> GHMQETQAVEAGEKTVEQFVQALNKGDYNKAAEMTSKKAANKSALSEKEILDKYQNIYGAADVKGLQISNLKVDKKDDSTYSFSY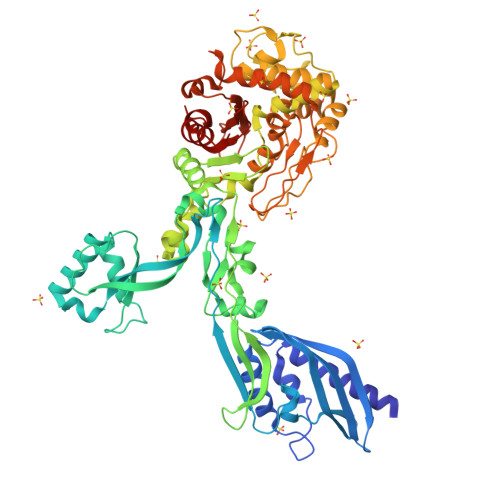KAKMNTSLGELKDLSYKGTLDRNDGQTTINWQPNLVFPEMEGNDKVSLTTQEAARGNIIDRNGEPLATTGKLKQLGVVPSKLGDGGEKTANIKAIASSFDLTEDAINQAISQSWVQPDYFVPLKIIDGATPELPAGATIQEVDGRYYPLGEAAAQLIGYVGDITAEDIDKNPELSSNGKIGRSGLEMAFDKDLRGTTGGKLSITDADGVEKKVLIEHEVQNGKDIKLTIDAKAQKTAFDSLGGKAGSTVATTPKTGDLLALASSPSYDPNKMTNGISQEDYKAYEENPEQPFISRFATGYAPGSTFKMITAAIGLDNGTIDPNEVLTINGLKWQKDSSWGSYQVTRVSSDVSQVDLKTALIYSDNIYAAQETLKMGEKKFRTGLDKFIFGEDLDLPISMNPAQISNEDSFNSDILLADTGYGQGELLINPIQQAAMYSVFANNGTLVYPKLIADKETKDKKNVIGETAVQTIVPDLREVVQDVNGTAHSLSALGIPLAAKTGTAEIKEKQDVKGKENSFLFAFNPDNQGYMMVSMLENKEDDDSATKRASELLQYLNQNYQ>MAEPQAESEPAAGGARGGGGDWPAGLTTYRSIQVGPGAAARWDLCIDQAVVFIEDAIQYRSINHRVDASSMWLYRRYYSNVCQRTLSFTIFLILFLAFIETPSSLTSTADVRYRAAPWEPPCGLTESVEVLCLLVFAADLSVKGYLFGWAHFQKNLWLLGYLVVLVVSLVDWTVSLSLVCHEPLRIRRLLRPFFLLQNSSMMKKTLKCIRWSLPEMASVGLLLAIHLCLFTMFGMLLFAGGKQDDGQDRERLTYFQNLPESLTSLLVLLTTANNPDVMIPAYSKNRAYAIFFIVFTVIGSLFLMNLLTAIIYSQFRGYLMKSLQTSLFRRRLGTRAAFEVLSSMVGEGGAFPQAVGVKPQNLLQVLQKVQLDSSHKQAMMEKVRSYGSVLLSAEEFQKLFNELDRSVVKEHPPRPEYQSPFLQSAQFLFGHYYFDYLGNLIALANLVSICVFLVLDADVLPAERDDFILGILNCVFIVYYLLEMLLKVFALGLRGYLSYPSNVFDGLLTVVLLVLEISTLAVYRLPHPGWRPEMVGLLSLWDMTRMLNMLIVFRFLRIIPSMKPMAVVASTVLGLVQNMRAFGGILVVVYYVFAIIGINLFRGVIVALPGNSSLAPANGSAPCGSFEQLEYWANNFDDFAAALVTLWNLMVVNNWQVFLDAYRRYSGPWSKIYFVLWWLVSSVIWVNLFLALILENFLHKWDPRSHLQPLAGTPEATYQMTVELLFRDILEEPEEDELTERLSQHPHLWLCR[2x]

Two-pore channel 2 (TPC2) is a nicotinic acid adenine dinucleotide phosphate (NAADP) and phosphatidylinositol-(3,5)-diphosphate (PI(3,5)P2)-activated Na+ and Ca2+-permeable channel in the endolysosomal system. Two pore channels are lysosomal cation channels with crucial roles in tumor angiogenesis and viral release from endosomes. High-resolution structures of mouse TPC1 and human TPC2 (HsTPC2) were recently determined with X-ray crystallography and cryo-electron microscopy (cryo-EM),35,36 where they showed homodimeric assembly of two subunits, each consisting of twelve transmembrane helices, resembling a tandem repeat of a 6 TM helices (6 TM I in N-terminal half and 6 TM II in C-terminal half) observed in voltage-gated ion channels (VGICs) of the Kv, Nav, and Cav families. Inhibition of the two-pore channel 2 (TPC2) has emerged as potential therapeutic strategy for the treatment of cancers and viral infections, including Ebola and COVID-19.

We determined the structure of HsTPC2 in complex with a pure (S)-enantiomer of a synthetic antagonist SG-094 with cryo-EM, where we uncovered not only the binding pocket and binding mode of the compound, further backed up by site-directed mutagenesis, patch-clamp experimentation, and Ca2+ imaging analysis, but also its influence on TPC2 conformation. We identified a sub-state of HsTPC2 with significant movement of VSD II domains, and refinement of this set of particles yielded a HsTPC2/SG-094 complex structure at 3.0 Å nominal resolution. Interestingly, VSD II domain of the other subunit in the homodimer does not show such a feature, which suggests an asymmetric binding of (S)-SG-094 to HsTPC2 with 1:1 dimer-to-ligand stoichiometry instead of 1:2 which would be expected with a full occupancy (the subunit with (S)-SG-094 will be referred to as subunit A, and the one without inhibitor will be referred to as subunit B). (S)-SG-094 is located at a cleft between IIS1 and IIS4 helices of VSD II on the cytoplasmic side near IIS4/5 linker helix. The compound lacks a polar interaction, and it mainly forms hydrophobic interactions with nearby residues, such as Y436, F555, and I558. At the local level, (S)-SG-094 triggers several side chains to reposition, creating a binding pocket which is absent in the 2-fold symmetrical apo state structure. On the other hand, SG-094 binding to VSD II induces a shift of IIS4 helix toward the cytoplasmic (i.e., C-terminal) side by one full turn, which results in Y480 interacting with I551 (R3) instead. The cytoplasmic shift of IIS4 helix in subunit A and associated movement of residues M562 and K563 lead to the stabilization of II S4/5 linker helix in a closed state with an extra helical turn on its N-terminal side. Therefore, it can be postulated that the binding of (S)-SG-094 in one subunit leads to the closure of its binding pocket in the other subunit, explaining the asymmetric binding of the compound to HsTPC2 homodimer.>PKALIVYGSTTGNTEYTAETIARELADAGYEVDSRDAASVEAGGLFEGFDLVLLGCSTWGDDSIELQDDFIPLF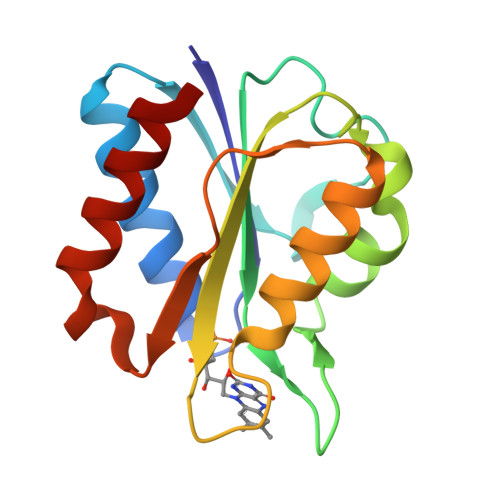DSLEETGAQGRKVACFGCGESSYEYFCGAVDAIEEKLKNLGAEIVQDGLRIDGDPRAARDDIVGWAHDVRGAI[2x]>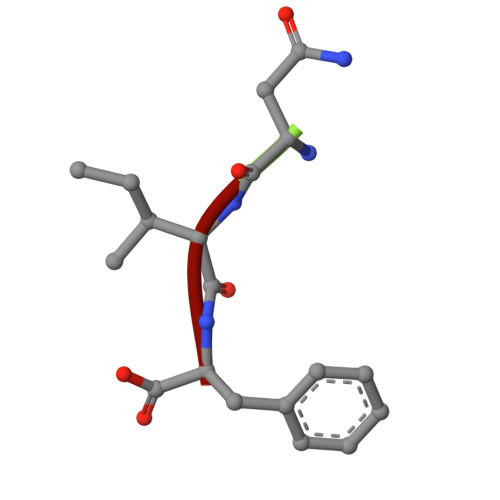 NIF> NLFQFGDMILQKTGKEAVHSYAIY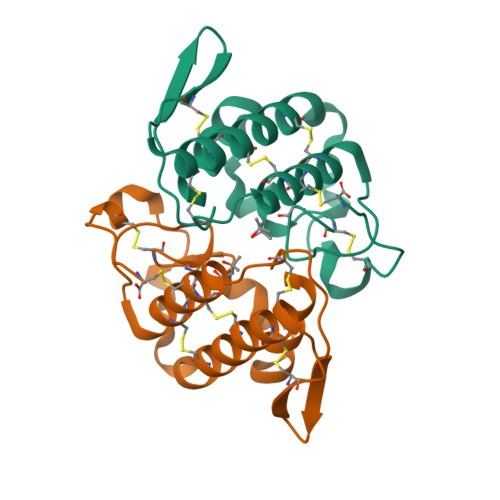GCYCGWGGQARAQDATDRCCFAQDCCYGRVNDCNPKTATYTYSFENGDIVCGDNDLCLRAVCECDRAAAICLGENVNTYDKNYEYYSISHCTEESEQC;> NLFQFAKMINGKLGAFSVWNYISYGCYCGWGGQGTPKDATDRCCFVHDCCYGRVRGCNPKLAIYSYSFKKGNIVCGKNNGCLRDICECDRVAANCFHQNKNTYNKNYKFLSSSRCRQTSEQC>SGPGFDFAQAIMKKNTVIARTEKGEFTMLGVYDRVAVIPTHASVGETIYINDVETKVLDACALRDLTDTNLEITIVRLDRNQKFRDIRHFLPRYEDDYNDAVLSVHTSKFPNMYIPVGQVTNYGFLNLGG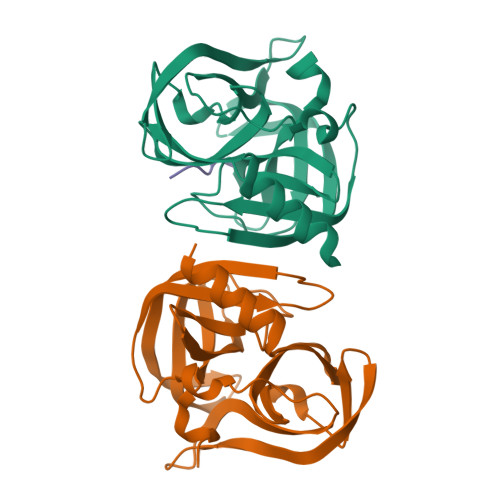TPTHRILMYNFPTRAGQAGGVVTTTGKVIGIHVGGNGAQGFAAMLLHSYFSD[2x];> AKVQGP> MNFDYMFKLLIIGNSSVGKTSFLFRYADDTFTPAFVSTVGIDFKVKTVYRHEKRVKLQIWDTAGLERYRTITTAYYRGAMGFILMYD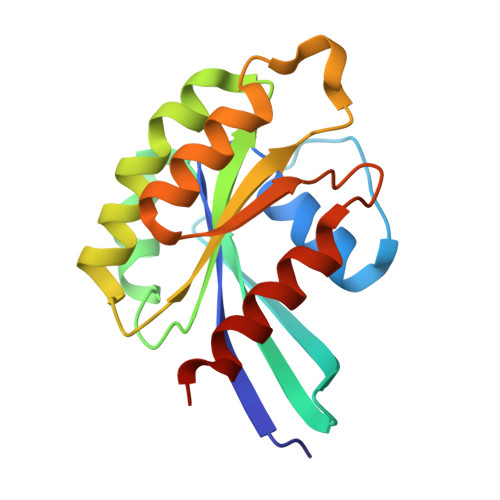ITNEESFNAVQDWATQIKTYSWDNAQVILVGNKCDMEEERVVPTEKGQLLAEQLGFDFFEASAKENISVRQAFERLVDAICDKMSDS1-METHYL ETHYL 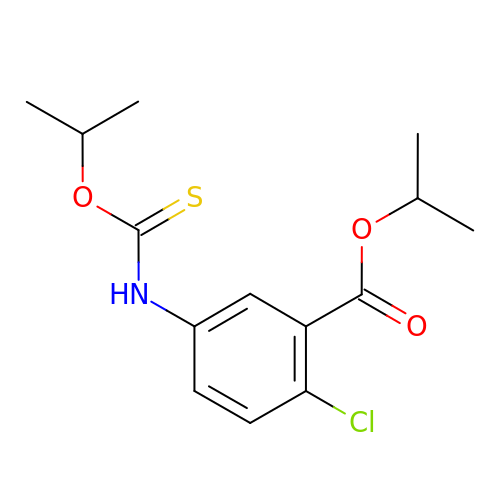2-CHLORO-5-[[[(1-METHYLETHOXY)THIOOXO]METHYL]AMINO]-BENZOATE | C14 H18 Cl N O3 S | AXTNFJKQZPETJA-UHFFFAOYSA-N benzimidazol-1-ylmethanol 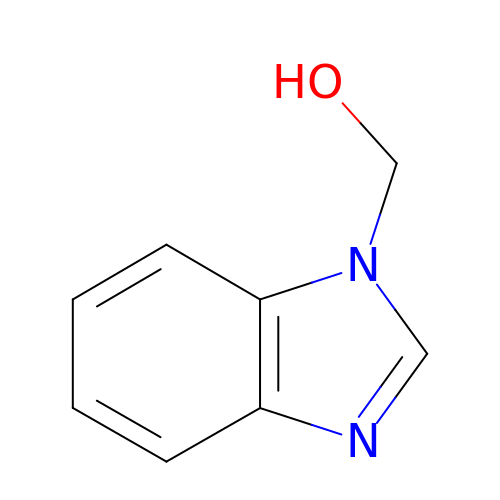| C8 H8 N2 O | IWCRZZKSGBFRSJ-UHFFFAOYSA-N> GGSPDKEVHLILYHWTHSFSSQKVRLVIAEKALKCEEHDVSLPLSEHNEPWFMRLNSAGEVPVLVHGENIICEATQIIDYLEQTFLDERTPRLMPDEGSMYYPRVQHYRELLDSLPMDAYTHGCILHPEGTGDNVKYLKKILD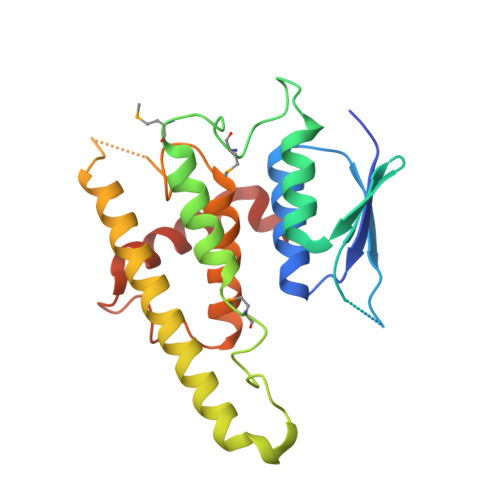ELEKVLDQVETELQRRNEETPEEGNQPWLCGESFTLADVSLAVTLHRLKFLGFARRNWGHGKRPNLETYYERVLKRKTFNKVEFGS> SNQLISNYAASNSMDRSSSASNEFVPNTSDNNNNSNNHNMRNNSNNKTSNNNNVTAVPAATPANTNNSTSNANTVFSERAAMFAALQQKQQQRFQALQQQQQQQQNQQQQNQQPQQQQQQQQNPKFLQSQRQQQQRSILQSLNPALQEKISTELNNKQYELFMKSLIENCKKRNMPLQSIPEIGNRKINLFYLYMLVQKFGGADQVTRTQQWSMVAQRLQISDYQQLESIYFRILLPYERHMISQEGIKETQAKRIFLQQFLQELLKKVQQQQQAAALANANNNINSASSAPTPAAPGASVPATAAPGTEAGIVPVSANTPKSLNSNININVNNNNIGQQQVKKPRKQRVKKKTKKELELERKEREDFQKRQQKLLEDQQRQQKLLLETKLRQQYEIELKKLPKVYKRSIVRNYKPLINRLKHYNGYDINYISKIGEKIDSNKPIFLFAPELGAINLHALSMSLQSKNLGEINTALNTLLVTSADSNLKISLVKYPELLDSLAILGMNLLSNLSQNVVPYHRNTSDYYYEDAGSNQYYVTQHDKMVDKIFEKVNNNATLTPNDSNDEKVTILVDSLTGNQLPTPTPTEMEPDLDTECFISMQSTSPAVKQWDLLPEPIRFLPNQFPLKIHRTPYLTSLKKIKDEIDDPFTKINTRGAEDPKVLINDQLSTISMILRNISFSDNNSRIMSRNFYLKRFISDLLWLVLIHPENFTCNRKILNFKKDLVIVLSNISHLLEIASSIDCLLILILVISFGQPKLNPMASSSSFGSESLTFNEFQLQWGKYQTFGVDILAKLFSLEKPNLNYFKSILLNKNTGN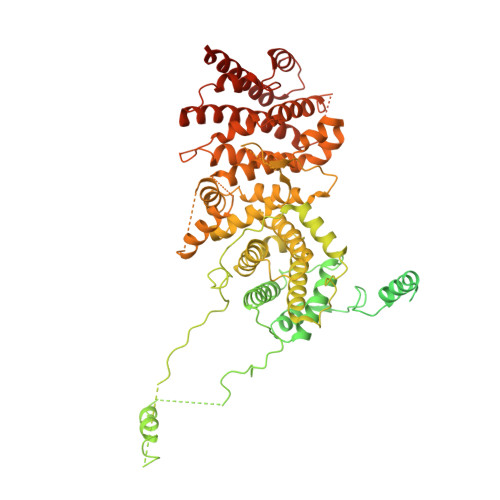NLYDRNSNNNHKDKKLLRRLLNLYNDNNKNNNNRHNLLNDVVSFLFSAIPLQQVLSQSADPSLLIDQFSPVISQSLTSILVIVQKILPLSNEVFEISENNSDSNSNNNGNKDSSFNFNKNLPFVWLSSEENIGSGLLKLSEIILNINNSTSKNTLLQQQNYSKVLLPSINISCVQLIKCLVEKSICFENCLNNDPEILKKIASIPNLFPTDLEIFQLFTNPSVDIQIINQYQLLYNLKNDILTNLEGGSGGWSHPQFEKWSHPQFEKWSHPQFEK> MKLPTNLAYERSIDPSDVCFFVVWPDDRKTPLTYNSRTLLGQMEAASLAYDVSGQPIKSATAEALAQGNPHQVDFCHVPYGASHIECSFSVSFSSELRQPYKCNSSKVKQTLVQLVELYETKIGWTELATRYLMNICNGKWLWKNTRKAYCWNIVLTPWPWNGEKVGFEDIRTNYTSRQDFKNNKNWSAIVEMIKTAFSSTDGLAIFEVRATLHLPTNAMVRPSQVFTEKESGSKSKSKTQNSRVFQSTTIDGERSPILGAFKTGAAIATIDDWYPEATEPLRVGRFGVHREDVTCYRHPSTGKDFFSILQQAEHYI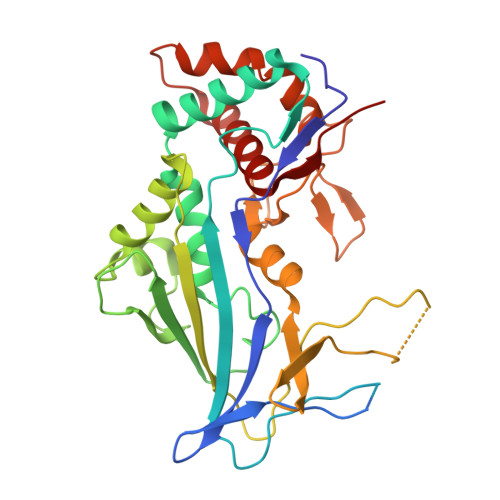EVLSANKTPAQETINDMHFLMANLIKGGMFQHKGD>[8x]LPSGSDPAFSQPKSVLDAGLTCQGASPSSVSKPILLVPGTGTTGPQSFDSNWIPLSTQLGYTPCWISPPPFMLNDTQVNTEYMVNAITALYAGSGNNKLPVLTWSQGGLVAQWGLTFFPSIRSKVDRLMAFAPDYKGTVLAGPLDALAVSAPSVWQQTTGSALTTALRNAGGLTQIVPTTNLYSATDEIVQPQVSNS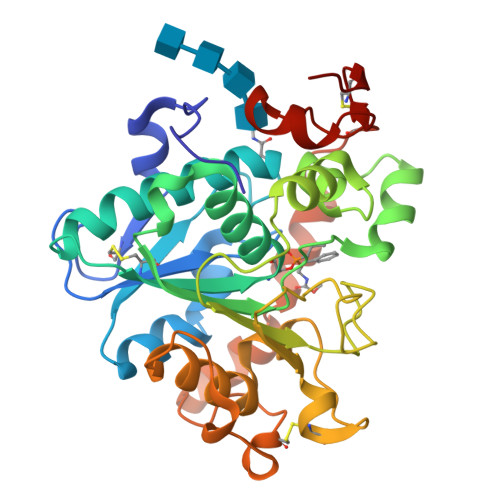PLDSSYLFNGKNVQAQAVCGPLFVIDHAGSLTSQFSYVVGRSALRSTTGQARSADYGITDCNPLPANDLTPEQKVAAAALLAPAAAAIVAGPKQNCEPDLMPYARPFAVGKRTCSGIVTP> MSPVLTTPKRHAPPPEQLQNVTDFNYTPSHQKPFLQPQAGTTVTTHQDIKQIVEMTLGSEGVLNQAVKLPRGEDENEWLAVHCVDFYNQINMLYGSITEFCSPQTCPRMIA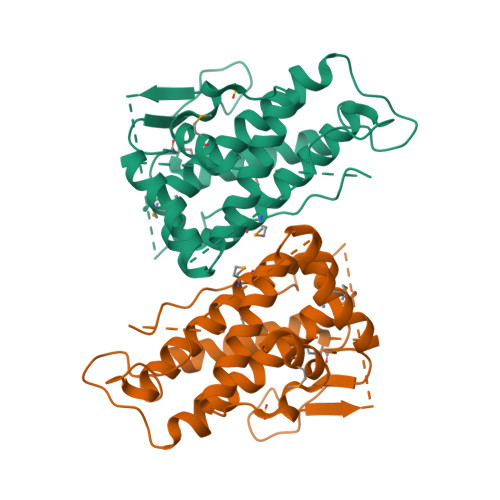TNEYEYLWAFQKGQPPVSVSAPKYVECLMRWCQDQFDDESLFPSKVTGTFPEGFIQRVIQPILRRLFRVYAHIYCHHFNEILELNLQTVLNTSFRHFCLFAQEFELLRPADFGPLLELVMELRDR4-[(3~{R})-3-(cyclobutylmethylamino)piperidin-1-yl]-1-[(1~{R})-1-[4-(5-methoxypyridin-3-yl)-1,2,3-triazol-1-yl]ethyl]pyridin-2-one | C25 H33 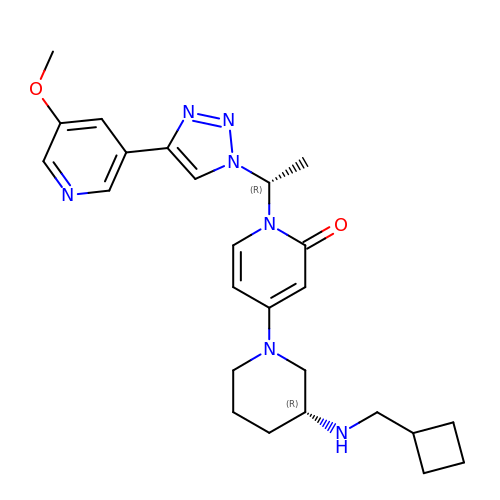N7 O2 | BLQHZTVKQVIIIR-WIYYLYMNSA-N> MASMTGGQQMGRDPNSMTNTLVENIY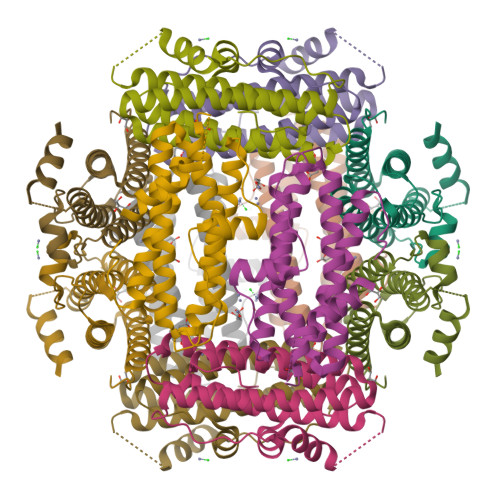ASVTHNISKKEASKNEKTKAVLNQAVADLSVAASIVHQVHWYMRGPGFLYLHPKMDELLDSLNANLDEVSERLITIGGAPYSTLAEFSKHSKLDEAKGTYDKTVAQHLARLVEVYLYLSSLYQVGLDITDEEGDAGTNDLFTAAKTEAEKTIWMLQAERGQGPALLEHHHHHH> XGEAAAA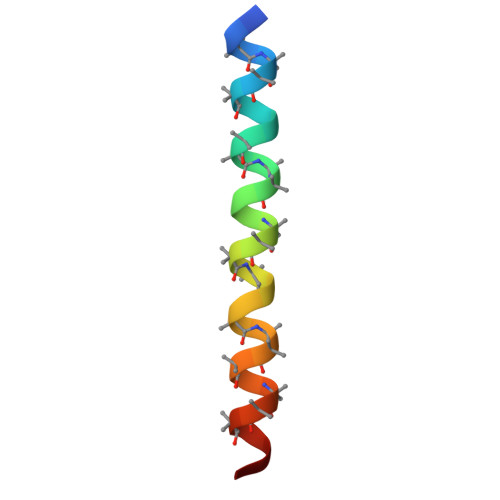KEAAAAKEAAAAKEAAAAKAAAWKGX> MGSSHHHHHHSSGRENLYFQGHMMNGDQNSDVYAQEKQDFVQHFSQIVRVLTEDEMGHPEIGDAIARLKEVLEYNAIGGKYNRGLTVVVAFRELVEPRKQDADSLQRAWTVGWCVELLQAFFLVADDIMDSSLTRRGQICW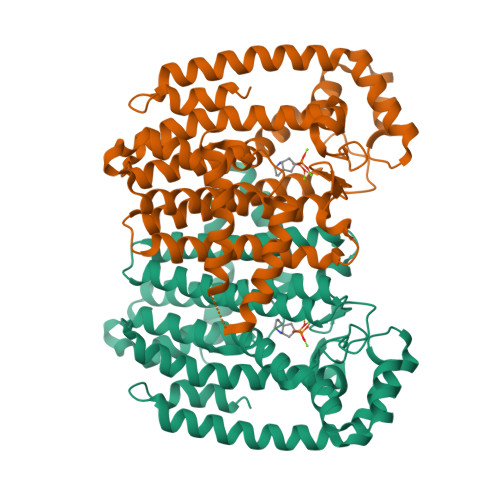YQKPGVGLDAINDANLLEACIYRLLKLYCREQPYYLNLIELFLQSSYQTEIGQTLDLLTAPQGNVDLVRFTEKRYKSIVKYKAAFYSFYLPIAAAMYMAGIDGEKEHANAKKILLEMGEFFQIQDDYLDLFGDPSVTGKIGTDIQDNKCSWLVVQCLQRATPEQYQILKENYGQKEAEKVARVKALYEELDLPAVFLQYEEDSYSHIMALIEQYAAPLPPAVFLGLARKIYKRRK>GAMADDIRILMCPPDHYDVDYVINPWMEGNIHKSSQERAVEQWKKLHQTIKECAIVDLVKPAKGWPDMVFTANAGLVLGENVVLSRFYHKERQGEEPYFKAWFEENGFTVYELPQDLPFEGAGDALFDREGRWLWAGYGFRSELDSHPYIAKWLDTEVVSLRLIDERFYHLDTCFCPLSGGYLLYYPPAFDAYSNRVIEMRIPPEKRIIVEELDAVNFACNAVNVNDIIIMNLVSRTLKEKLAEAGFKVRETPLTEFLKAGGAAKCLTLRVTEPILPDVHATVSIESRVIRMEGHLLDAGILNQALDLVVENSGSFRVLNFNLGVERNSTSSAEVRVSAPSHQIMEEIMTELIDLGAVPPPQELCDINTETVTQGGVAPDDFYVSTIYPTEVRVNCEWVQVTG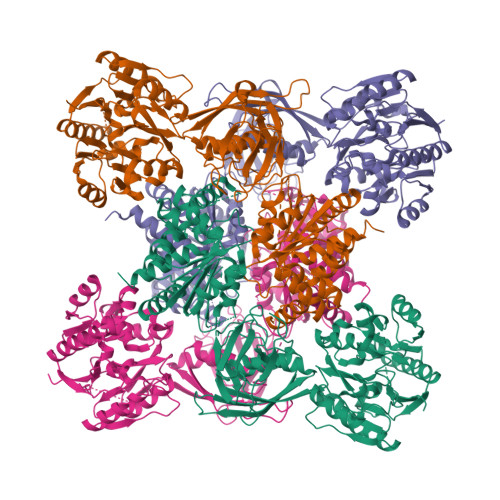QRMDAAIVVTSNPPSARCVLLRDLQVGDRVMVGVEGIRTIKKVESHEGGTRKENKEFAFMAAGVSSERRVELLVEQIAWEMRQIRDQGGKIVVTAGPVVIHTGGAQHLSHLVREGYVHALLGGNAIAVHDIEQATMGTSLGVDMQRGIPVRGGHRHHLKIINSVRRYGGIRQAVEAGFISKGVMYECVKNNIPYCLAGSIRDDGPLPDTEMNLVRAQSRYSELIQGADMILMLSSMLHSIGVGNMTPSGVKMVCVDINPAVVTKLSDRGSVESVGVVTDVGLFLSLLVRQLQQLTRPYSLAETL[4x]>MEKKALTLAERQ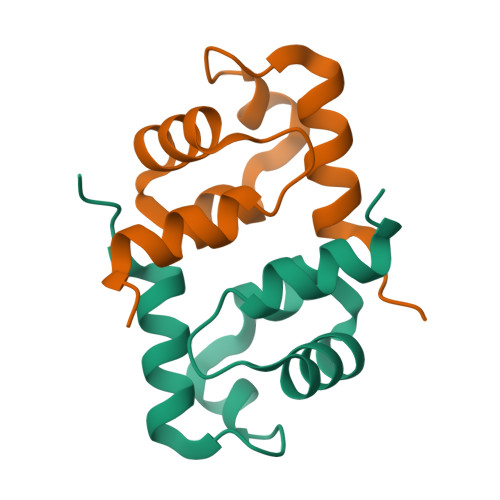RLIVEGLPHVSATLARRLLKHFGSVERVFTASVAELMKVEGIGEKIAKEIRRVITAPYIEDEE[2x]> AAGGYVALGDSYSSGVGAGSYDSGSGDCRRTPKAYPALWAAANSPASFDFVACSGAVTSDVLNKQMGPLNSSTSLVSLTIGGNDAGFADVMTTCVLQSEANCIARVNTAKAFVESTLPGRLDSVYSQVRAKAPSANVVVLGYPRFYKLNGTCVAGLTEGERTAINGAADLLNSVISKRAADHGYAYGDIAAAFTGHEICSGDSWLHS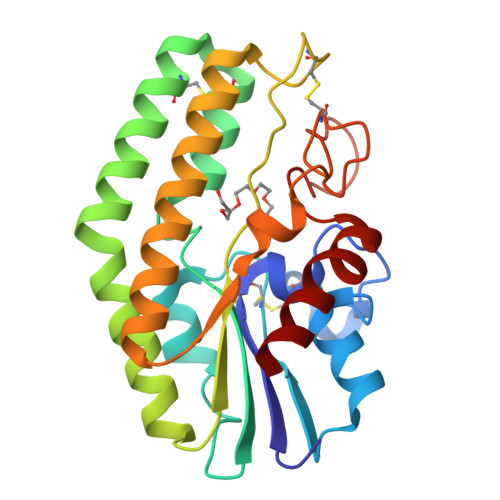VKWTGINDSYHPTAAGQSGGYLPVLNSKA> GHMAVIKVIGVGGGGGNAVEHMVRERIEGVEFF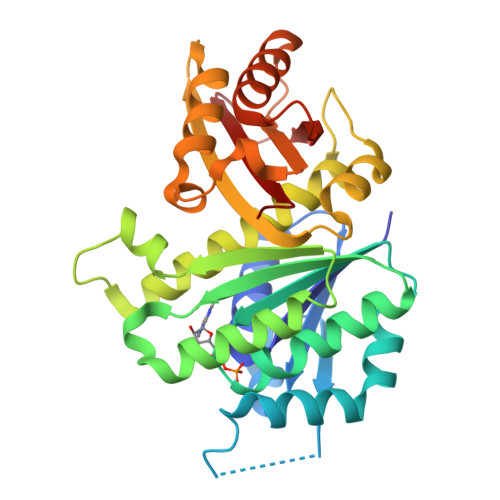AVNTDAQALRKTAVGQTIQIGSGITKGLGAGANPEVGRNAADEDRDALRAALEGADMVFIAAGMGGGTGTGAAPVVAEVAKDLGILTVAVVTKPFNFEGKKRMAFAEQGITELSKHVDSLITIPNDKLLKVLGRGISLLDAFGAANDVLKGAVQGIAELITRPGLMNVDFADVRTVMSEMGYAMMGSGVASGEDRAEEAAEMAISSPLLEDIDLSGARGVLVNITAGFDLRLDEFETVGNTIRAFASDNATVVIGTSLDPDMNDELRVTVVATGIG The PIN (PilT N-terminus) domain is a small domain with ~ 130 amino acid residues and is widely distributed in all three kingdoms of life. The activity of PIN domain depends on four conserved acidic residues and the presence of Mn2+ or Mg2+ ion. Utp24 is the endonuclease proposed to cleave the A1 and A2 sites. Depletion of Utp24, aka Fcf1 (Faf1 copurifying factor 1), inhibits cleavage at sites A0, A1 and A2 in yeast, whereas mutations of the active site of Utp24 specifically block cleavage at sites A1 and A2, but not at site A0. This suggests that Utp24 plays both a structural and catalytic role in 90S.

In this study, we determined a crystal structure of the PIN domain of Utp24 from Schizosaccharomyces pombe. The crystal belongs to space group C2221 and contains one molecule in the asymmetric unit. The structure was determined with molecular replacement using the Utp23 structure as search model and refined to an Rfree/Rwork of 0.287/0.222 at 2.14 Å resolution. Although the full-length protein of spUtp24 was used in crystallization, the crystal structure contains only the PIN domain (residues 60–192). The N-terminal region was not resolved likely due to flexibility or degradation. The structure adopts a compact three-layer fold with a mixed six-strand β-sheet packed by helices α1-α4 at one side and helices α5 and α6 at the other side. A zinc ion is coordinated with Cys103, Cys132, His134 and Cys142, which are invariant in Utp24 orthologues. PIN domains contain commonly four acidic residues required for catalysis. These residues, Asp70, Glu107, Asp140 and Asp159 in spUtp24, are clustered at the N-termini of helices α1, α5 and α6 and the middle of helix α3. The spUtp24 structure is well aligned to the recently determined cryo-EM structures of S. cerevisiae and C. thermophilum Utp24 (scUtp24 and ctUtp24) in 90S with RMSD = 0.86–0.98 Å.

> SLGPPYHVIIDTNFINFCLQQKIDLFEGLMTCLYAKTIPCISDCVMAELEKLGIRYRIALRIAKDERFERLPCTHKGTYADDCIVQRVMQHKCYLVATNDKNLKQRIRKIPGIPILSVANHKIRVERLVDVVD>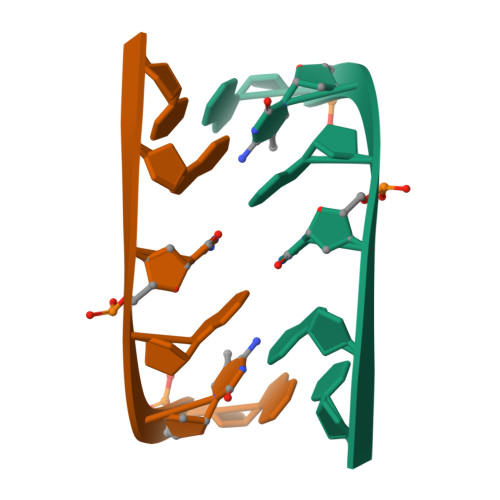[2x]GCGCGC> GMQEHYQPAAIEPAAQKKWDDARISNVSEDASKPKYYCLSMFPYPSGKLHMGHVRNYTIGDVLSRFKLLNGFNVMQPMGWDAFGMPAENAAMKNNVAPAAWTYDNIEYMKTQLKSLGFAVDWEREVATCKPEYYRWEQWLFTKLFEKGIVYRKNGTVNWDPVDQTVLANEQVIDGRGWRSGALIEKREIPMYYFKITDYAEELLNDLDKLEHWPEQVKTMQRNWIGKSRGMTVRFAVSDDSKQGLEGDYAKFLQVYTTRPDTLMGATYVAVAAEHPLATAAAADKPELQAFIAECKAGSVAEADMATMEKKGVPTGRYVVNPLNGDKLEVWIANYVLWGYGDGAVMAVPAHDERDFEFAAKYNLPKKQVIAVGDNAFDANRWQEWYGDKENGVLVNSGDLDGLDFQTAFDAVAAKLQSQGAGEPKTQYRLRDWGISRQRYWGCPIPIVHCEKCGNVPVPADQLPVVLPENVVPDGMGSPLAKMPEFYETSCPCCGGAAKRETDTMDTFIESSWYFFRYMSPKFSDGMVSAESAKYWGAVDQYIGGIEHAIGHLLYARFFTKLMRDEGLVNVDEPFERLLTQGMVVCETYYRENDKGGKDWINPADVELTFDDKGRPVSAVLKADGLPVVISGTEKMSKSKNNGVDPQELINAYGADTARLFMMFAAPPEQSLEWSDSGVEGAHRFLRRLWRTVYEYLKQGGAVKA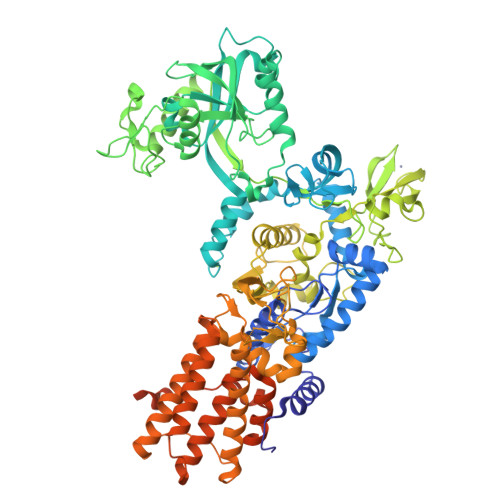FAGNQDGLSKELKDLRHKLHSTTAKVSDDYGRRQQFNTAIAAVMELLNQYDKTDTGSEQGRAVAQEVLEAAVRLLWPIVPHICETLWSELNGAKLWEAGWPTVDEAALVKSEIEVMVQVNGKLRGKITVAADASKADLEAAALANEGAVKFMEGKPAKKIIVVPGRLVNIVV>[2x]MSSCKDSLSLMAMWGSIARFDPKHERSFEGPEKRLEVIMRVVDGTHVSGLLAHDDDVWQKVIDAICAHIVSREFNEYIRSYVLSE;>[2x]XSLFVMKDRVILITCGTITLLNCVPLICEAVSTVCGEVEWVSFMHKNYSFPWEQKGPHLSMAEEFKTLRSHFPSGQPFIFGPIDSDHYFLYFHSDVVQPSCSDDAQLSMTMYGLDRNQTKHWYSDKMLPTGPETAVIREATGLSEVVDDSWILHDLQYEPCGYSINAIRGSEYQTIHITPEEHCSFASYETNTCALNYSKCICGVLRVFDPERFSVIVFIDPDSAVGKSYHSGGTIGVEPEYYPNYEAHHRTVNEYTPGHWVLKVNYVKRAVGTVGTSAASGAKE;>[2x]MSVTRINQQTECPSSVHDLVSCWGGCTQSKTSTDSGLEKRFELNFAQPVDIGTVTVKQLASVMERAGESLRQNSAELGIHTLKFDRSLLVFTAKQIVVRSSVSVMLHEAVHPMLELMRSHNIIVDWASFMRVNYGSPWDMTSETSDIMAHEYAELKSAFPTGHPYLAGPVDRDHCFYFVYDGIDRDPSSCRRENDVQINVYMYNVQADDEYDLDGNTKEQQLLVSHCAGEYETLRVSTYGSTHPFASFETNAVSAASDITKIVNGLLKKFYPERVLLVLLQDRDAQGTTACGVMDRLEGFTVVHRGANHFGGGYVFHQATYARSA

AdoMetDC is a pyruvoyl-dependent enzyme that catalyzes formation of decarboxylated AdoMet, a substrate required for biosynthesis of the polyamine spermidine from putrescine. The AdoMetDC pyruvoyl group plays a key role in the catalytic mechanism and derives from an autocatalytic processing reaction that cleaves the peptide backbone into β- and α-chains. Trypanosomatid AdoMetDC undergoes this cleavage, while the corresponding pseudoenzyme, which we call ‘prozyme’, lacks key residues and is not processed to the active form.

TbAdoMetDC/prozyme wild-type heterodimer was crystallized with putrescine both in the absence (apo-TbAdoMetDC/prozyme) and presence (CGP-TbAdoMetDC/prozyme) of CGP 40215 (CGP), a known AdoMetDC inhibitor. Crystals (space group P21) from both conditions diffracted to 2.4 Å. Two TbAdoMetDC/prozyme heterodimers are observed per asymmetric unit. They are associated in a tetrameric structure formed partially through a domain swap involving prozyme β-strands (β0’), but which buries a relatively small surface area. The TbAdoMetDC/prozyme complex was previously shown to be a dimer in solution by analytical ultracentrifugation, thus the tetramer is unlikely to be relevant to its catalytic function. In prozyme, the electron density is consistent with a bound putrescine (Put’); however, in TbAdoMetDC the corresponding electron density is larger and the crystallization buffer bis-tris propane (B3P) was modeled into the site. The TbAdoMetDC/prozyme dimer interface contains an extensive buried surface area (3,200 Å2). Strands β9-β16 form a scaffold that extends across the dimer interface with H-bond interactions formed between β15 from TbAdoMetDC (R336-E340) and β15’ from prozyme (R305-H309). Firstly, in the TbAdoMetDC/prozyme heterodimer, the autoinhibitory residues (S27-G30) have been displaced from the active site, which relieves the autoinhibition and positions F28 to form the catalytically competent ligand-binding site. This movement is facilitated by cis-to-trans isomerization of P31.>[2x]GAMDPEFMELRVGNRYRLGRKIGSGSFGDIYLGTDIAAGEEVAIKLECVKTKHPQLHIESKIYKMMQGGVGIPTIRWCGAEGDYNVMVMELLGPSLEDLFNFCSRKFSLKTVLLLADQMISRIEYIHSKNFIHRDVKPDNFLMGLGKKGNLVYIIDFGLAKKYRDARTHQHIPYRENKNLTGTARYASINTHLGIEQSRRDDLE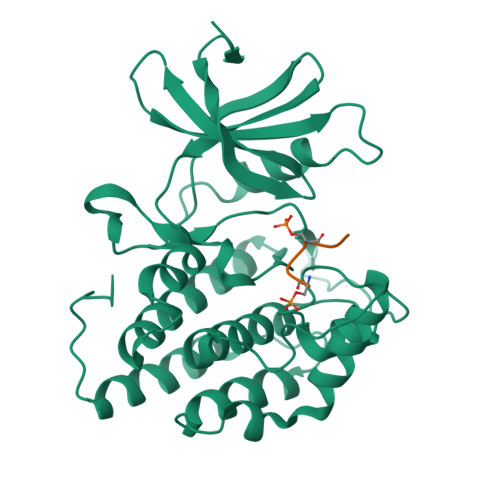SLGYVLMYFNLGSLPWQGLKAATKRQKYERISEKKMSTPIEVLCKGYPSEFATYLNFCRSLRFDDKPDYSYLRQLFRNLFHRQGFSYDYVFDWNMLK;>GKAESVASLT[2x]> MGCQSTQLQTPAPDTGGIVELNRQLGRGVNLGNALEAPWEGAWGVRLEEGFFELIREAGFKTIRLPVSWTHHAGRAAPYTIDPAFFSRVDWAVTQATRRGLNIVVNVHHYDELNANPQAEE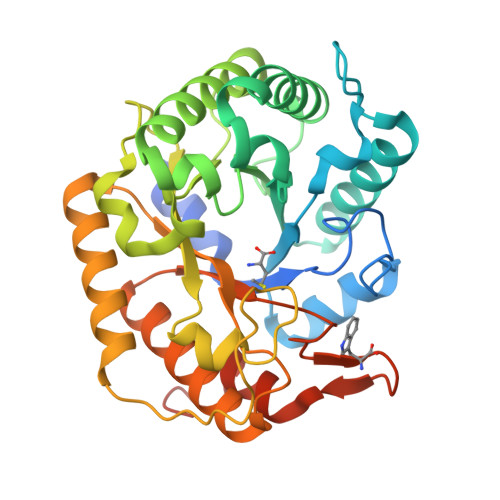ARYLSIWRQIAERYRNQPGSVYFELLNEPHGRFNDNPQLWNDLLAKALRVVRESNPSRAVIVGPVGWNSLWRLSELRLPDDPNLIVTFHYYDPLEFTHQGAEWLNPVPPTGVVWHQQNAIAQAMEFAQRWAEQNRRPIFVGEFGAYEKGDLDSRVRWTGAVRSELEKRNFSWAYWEFAAGFGIYDRTTRQWRTPLLKALVPEQPKLKLAAALEHHHHHH> AIQTRA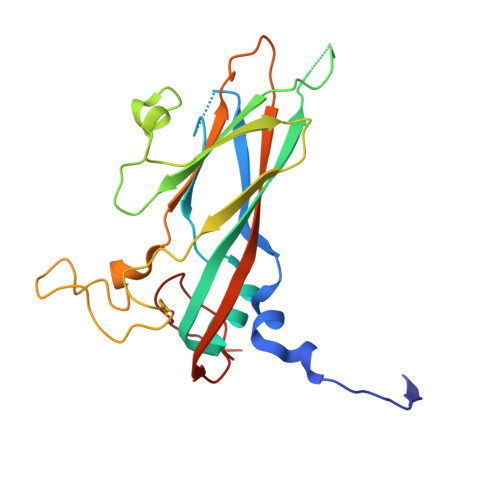VINQHGTSETLVENFLGRAALVMMKDFEYKNHVTGTQKVQQNFFKWTINTRSYVQLRRKFELFTYIRFDSEITIVPTIRLYTSTGASYSGLPNLTLQAMFVPVGAPTPKSQDSYEWQSACNPSVFFKIDDPPARMTIPFMCINSAYGMFYDGFAGFEKTANGLYGINPANTMGNLCIRVVNAYQPVQYTITIRIYLKPKHIKAWVPRPPRTMPYMSIANTNYTGH> MPYYAFAEPFFIHAITHLHVGSGSSVEEEIALPFQRDELGYPTIYASSLKGAIKSFLLKEFPDKRDVIYKVLGEDENPEEASLGTFLDAILFAIPSRIIEIDSAKPYVWVYVTTYELLKKVKLYLDSISQLSNASFSNL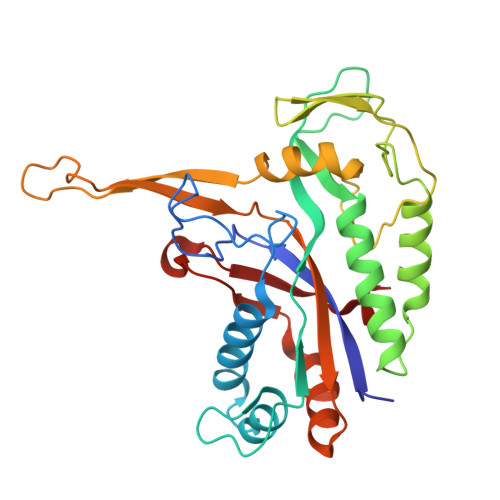KNKIDTILAKEGKNITLDSDLKSAILNEDFYVELEALNNKIPSIINAGVPLLVLEDSIGREVINRSLIRVRRIRIDRDKKVVETGGLWSEEYVPMKTIFFSVLLGKESKESAIFASCILRNLRYVILGGKETIGKGIVELRWVKDVI> METDLNSQDRKDLDKFIKFFALKTVQVIVQARLGEKICTRSSSSPTGSDWFNLAIKDIPEVTHEAKKALAGQLPAVGRSMCVEISLKTSEGDSMELEIWCLEMNEKCDKEIKVSYTVYNRLSLLLKSLLAITRVTPAYRLSRKQGHEYVILYRIYFGEVQLSGLGEG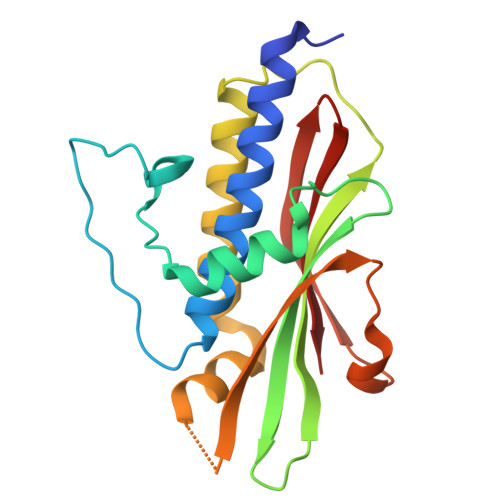FQTVRVGTVGTPVGTITLSCAYR>GPLGSLTMGAQDTLPVAAAFTETVNAYFKGADPSKCIVKITGEMVLSFPAGITRHFANNPSPAALTFRVINFSRLEHVLPNPQLLCCDNTQNDANTKEFWVNMPNLMTHLKKVSEQKPQATYYNVDMLKYQVSAQGIQSTPLNLAVNWRCEPSSTDLRIDYKYNTDAMTTAVALNNVQFLVPIDGGVTKLQAVLPPAVWNAEQQRILWKIPDISQKSENGGVGSLLARFQLSEGPSKPSPLVVQFTSEGSTLSGCDIELVGAGYRFSLIKKRFAAGKYLADN[2x]

Src homology 3 (SH3)-domain growth factor receptor-bound 2-like (endophilin) interacting protein 1 (SGIP1) and its splicing variant, SGIP1α, are brain-specific homologs of FCHo1/FCHo2. The μHDs of SGIP1 and SGIP1α, which are identical to each other, are highly homologous to those of FCHo1/FCHo2. The μHD of SGIP1/SGIP1α also binds to the DPF motif-rich region of Eps1519. Thus, the SGIP1/FCHo1/FCHo2 μHD is a domain designed for recognizing the locally ordered structure formed by the two consecutive DPF motifs.

To gain further insights into the mechanism of DPF-motif recognition by the μHD, we solved the crystal structures of the SGIP1 μHD in two different space groups. The two structures are similar to each other, and the minor differences in the secondary structure composition are probably due to crystal packing effects. The structure of the SGIP1 μHD adopts a topology similar to those of the previously determined μHD structures. However, the SGIP1 μHD possesses unique structural features that distinguish it from the other known μHD structures. Among these distinctive features, the most prominent one is the presence of the SGIP1/FCHo1/FCHo2-specific insertion of a relatively long α-helix (α2) between β6 and β7. Due to this insertion, the loop between α2 and β7 and the N-terminal part of β7 also adopt conformations strikingly different from those in other μHDs. Since these regions contain critical Eps15 interacting residues (see below), these unique structural features of the SGIP1 μHD are functionally relevant.> MDDFASLPLVIEPADLQARLSAPELIL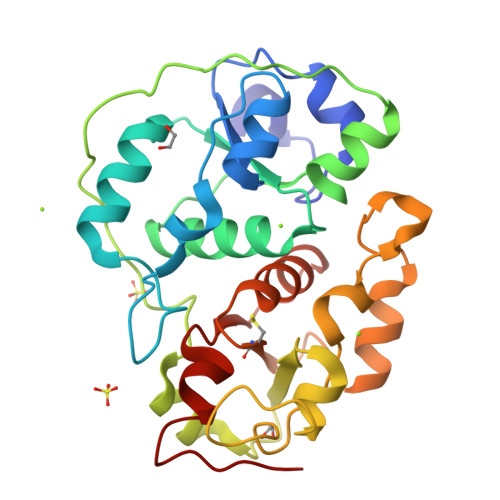VDLTSAARYAEGHIPGARFVDPKRTQLGQPPAPGLQPPREQLESLFGELGHRPEAVYVVYDDEGGGWAGRFIWLLDVIGQQRYHYLNGGLTAWLAEDRPLSRELPAPAGGPVALSLHDEPTASRDYLLGRLGAADLAIWDARSPQEYRGEKVLAAKGGHIPGAVNFEWTAAMDPSRALRIRTDIAGRLEELGITPDKEIVTHCQTHHRSGLTYLIAKALGYPRVKGYAGSWGEWGNHPDTPVEL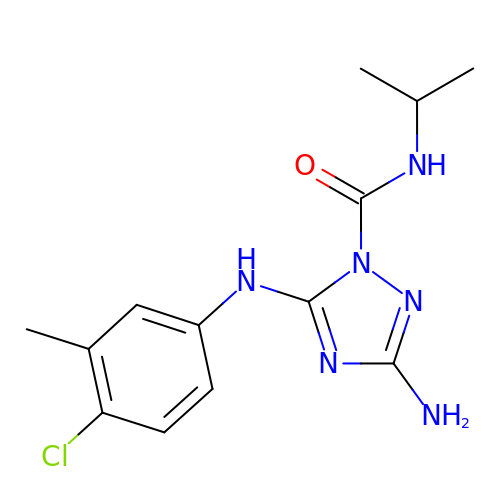3-amino-5-[(4-chloro-3-methylphenyl)amino]-N-(propan-2-yl)-1H-1,2,4-triazole-1-carboxamide | C13 H17 Cl N6 O | HSFMSVIZAIBADX-UHFFFAOYSA-N> MYGDLGNKLVLEAKRTKQLYARSNQDVNLPMYHEDIIRNILKEVSNLRKNTEYLKEQQQLGMLDDKVAKCQYFVTLLCMERNKRCLLAYQRLRTDILDSMAWNNNGLDLMSSITFSQQDTNNLSHQEQEYLKEYCD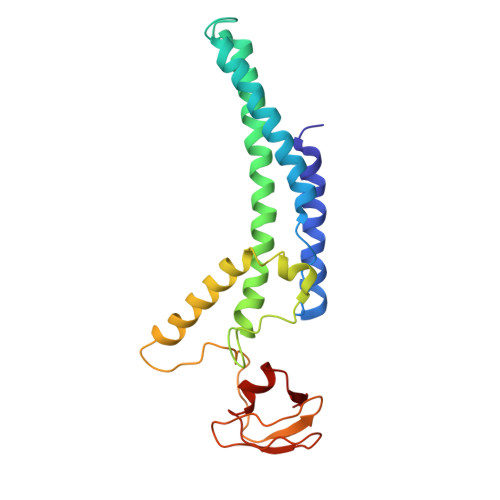LITDLKSGDLVDIDLSGSLVPPSDVFIDVRVLKDAGEIQTEYGVFNLIKDSQFFVRQSDVERLIQQGYLQKI N1-(5-(2-(6-Amino-4-methylpyridin-2-yl)ethyl)pyridin-3-yl)-N1,N2-dimethylethane-1,2-diamine 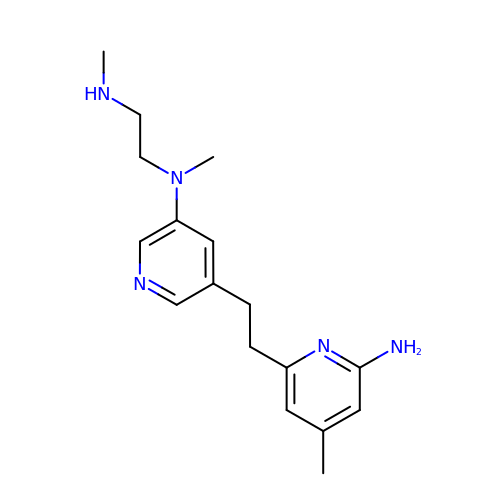| C17 H25 N5 | BAILAIZRWKFZJT-UHFFFAOYSA-N> ADPPAPSTRRPPAPNLHVSPELFCEPREVRRVQWPATQQGMLVERPCPKGTRGIASFQCLPALGLWNPRGPDLSNCTSPWVNQVAQKIKSGENAANIASELARHTRGSIYAGDVSSSVKLMEQLLDILDAQLQALRPIERESAGKNYNKMHKRERTCKDYIKAVVETVDNLLRPEALESWKDMNAT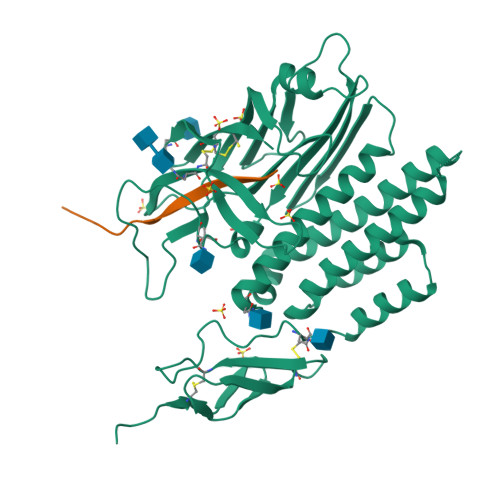EQVHTATMLLDVLEEGAFLLADNVREPARFLAAKQNVVLEVTVLSTEGQVQELVFPQEYASESSIQLSANTIKQNSRNGVVKVVFILYNNLGLFLSTENATVKLAGEAGTGGPGGASLVVNSQVIAASINKESSRVFLMDPVIFTVAHLEAKNHFNANCSFWNYSERSMLGYWSTQGCRLVESNKTHTTCACSHL;> TNFAVLMAHREIYHHHHH>[2x]AAAGGGG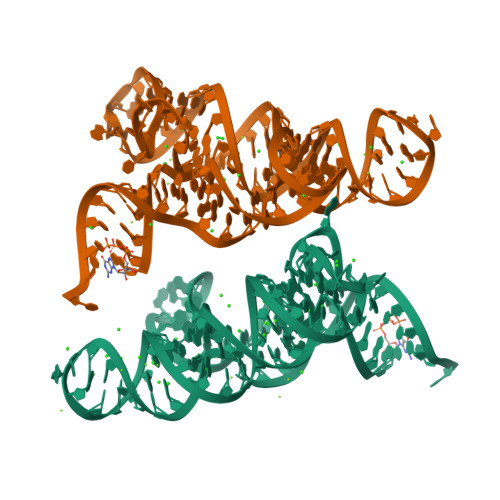AGUAGCGUCGGGAAACCGAAACAAAGUCGUCUAUUCGUGAGGAAACUCACCGGCUUUGUUGACAUACGAAAGUAUGUUUAGCAAGACCUUUCC>MSLATITNHMPTAELQALDAAHHLHPFSANNALGEEGTRVITRARGVWLNDSEGEEILDAMAGLWCVNIGYGRDELAEVAARQMRELPYYNTFFKTTHVPAIALAQKLAELAPGDLNHVFFAGGGSEANDTNIRMVRTYWQNKGQPEKTVIISRKNAYHGSTVASSALGGMAGMHAQSGLIPDVHHINQPNWWAEGGDMDPEEFGLARARELEEAILELGENRVAAFIAEPVQGAGGVIVAPDSYWPEIQRICDKYDILLIADEVICGFGRTGNWFGTQTMGIRPHIMTIAKGLSSGYAPIGGSIVCDEVAHVIGKDEFNHGYTYSGHPVAAAVALENLRILEEENILDHVRNVAAPYLKEKWEALTDHPLVGEAKIVGMMASIALTPNKASRAKFASEPGTIGYICRERCFANNLIMRHVGDRMIISPPLVITPAEIDEMFVRIRKSLDEAQAEIEKQ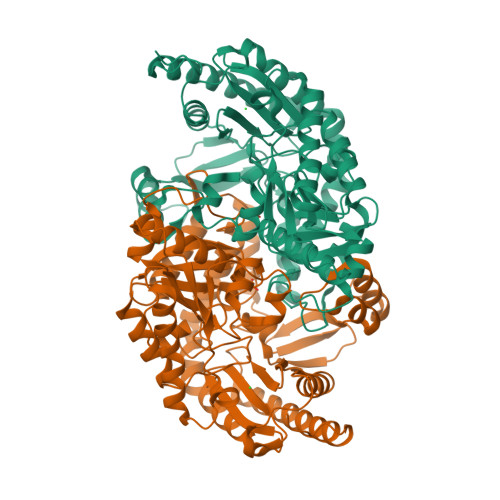GLMKSEGHHHHHH[2x]> HHHHHMAEQVKLSVELIACSSFTPPADVEWSTDVEGAEALVEFAGRACYETFDKPNPRTASNAAYLR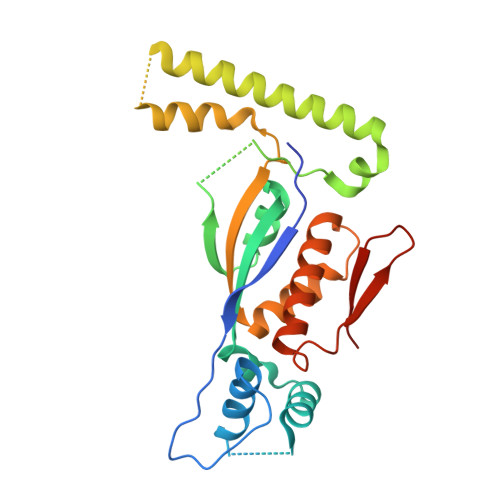HIMEVGHTALLEHANATMYIRGISRSATHELVRHRHFSFSQLSQRFVHSGESEVVVPTLIDEDPQLRELFMHAMDESRFAFNELLNALEEKLGDEPNALLRKKQARQAARAVLPNATESRIVVSGNFRTWRHFIGMRASEHADVEIREVAVECLRKLQVAAPTVFGDFEIETLADGSQMATSPYVMDF>MKSLQALFGGTFDPVHYGHLKKVETLANLIGLTRVTIIPNNVPPHRPQPEANSVQRKHMLELAIADKPLFTLDERELKRNAPSVTAQTLKEWRQEQGPDVPLAFIIGQDSLLTFPT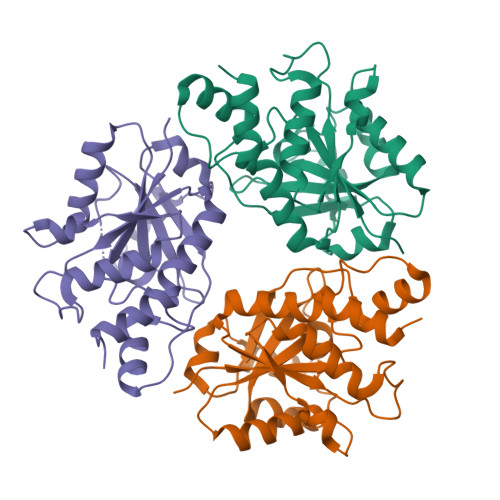WDEYETILDNAHLIVQRRPGYPLEMAQPQYQQWLEDHLTHNPEDLHLQPAGKIYLAETPFFNISATIIRERLQNGESCEDLLPEPVLTYINQQGLYR[6x]>MHHHHHHLEVLFQGPSSTVTIEYFNQKKEMTKTLEEITRDFEKENPKIKVKVVNVPNAGEVLKTRVLAGDVPDVVNIYPQSIELQEWAKAGVFEDLSNKDYLKRVKNGYAEKYAVNEKVYNVPFTANAYGIYYNKDKFEELGLKVPETWDEFEQLVKDIVAKGQTPFGIAGADAWTLNGYNQLAFATATGGGKEANQYLRYSQPNAIKLSDPIMKDDIKVMDILRINGSKQKNWEGAGYTDVIGAFARGDVLMTPNGSWAITAINEQKPNFKIGTFMIPGKEKGQSLTVGAGDLAWSISATTKHPKEANAFVEYMTRPEVMQKYYDVDGSPTAIEGVKQAGEDSPLAGMTEYAFTDRHL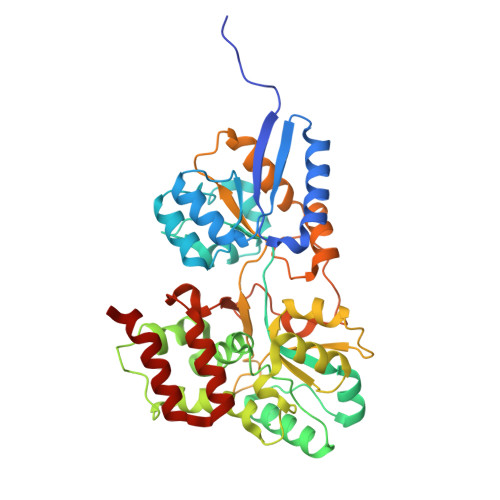VWLQQYWTSEADFHTLTMNYVLTGDKQGMVNDLNAFFNPMKM[3x]VanS is a sensor histidine kinase that responds to the presence of vancomycin by autophosphorylating and subsequently transferring the phosphoryl group to the response regulator, VanR. The phosphotransfer activates VanR as a transcription factor, which initiates the expression of resistance genes. The VanS sensor kinase is organized into several structural domains, which include a periplasmic sensor domain flanked by two transmembrane helices, a membrane-proximal HAMP domain, a dimerization-and-histidine-phosphorylation (DHp) domain, and a catalytic ATP-binding (CA) domain. Here, we present X-ray crystal structures for the catalytic and ATP-binding (CA) domains of two VanS proteins, derived from vancomycin-resistant enterococci types A and C. Both proteins adopt the canonical Bergerat fold that has been observed for CA domains of other prokaryotic histidine kinases.

The structure of the VanSC CA domain was determined by molecular replacement, using an ensemble of homology models as probes. The crystal asymmetric unit contains two copies of the CA domain, related by an approximate twofold axis of symmetry. The two protomers in the asymmetric unit are highly similar, with superposition yielding an RMSD for Cα positions of 0.25 Å (0.74 Å for all atoms). Metal ions also figure in the crystal packing of the VanSC protein, with 3 Mg2+ ions being situated in two different lattice interfaces. In particular, helix α3 occupies very different positions in the two structures, being positioned much closer to the nucleotide-binding site in VanSA than in VanSC. Hence, it seems likely that the ATP lids of VanSA and VanSC can adopt a range of positions, and crystallization of these two proteins has selected for two different conformers. The N291D VanSC CA domain was also less stable than its wildtype form, but we were able to express and purify sufficient quantities to perform binding studies. The mutant’s affinity for TNP–ATP was decreased relative to wildtype; unfortunately, the ATP competition assay could not be performed, as protein precipitated in the presence of high concentrations of ATP. We were able to perform equilibrium dialysis experiments with the mutant, but these assays showed no evidence of ATP binding. Finally, it is interesting to note that our two CA domains are derived from two different “flavors” of VRE, namely types A and C. Type A VRE exhibit inducible resistance to vancomycin, that is, cell wall precursors are not altered in the absence of the antibiotic; in contrast, many (but not all) type C VRE exhibit constitutive resistance, meaning that the resistance phenotype is observed in both the presence and absence of the antibiotic.

>LQTETTDLSLMLEQLTFEFLPLLEEKNLNWQLNLQKNVLATVDTEKIARVFDNLIRNAINYSYPDSPLLLELVESDSIHIRLTNRGKTIPEEMIGRLFEPFYRMDSSRATATSGTGLGLPIAKEILLASGGDISAESKDETIIFNVRLPKPANN[2x]>SFNPWFLTGFSDAECSFSILIQANSKYSTGWRIKPVFAIGLHKKDNELLKRIQSYLGVGKIHIHGKDSIQFRIDSPKELEVIINHFENYPLVTAKQADYTLFK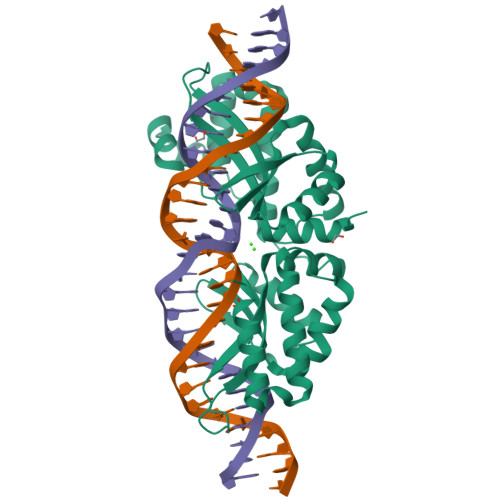KALDVIKNKEHLSQKGLLKLVGIKASLNLGLNGSLKEAFPNWEELQIDRPSYVNKGIPDPNWISGFASGDSSFNVKISNSPTSLLNKRVQLRFGIGLNIREKALIQYLVAYFDLSDNLKNIYFDLNSARFEVVKFSDITDKIIPFFDKYSIQGKKSQDYQNFKEVADIIKSKNHLTSEGFQEILDIKASMNK[2x]>[4x]MVSAPSIDTPSATTFDFDSSVFKKEKVTLSGHDEYIVRGGRNLFPLLPDAFKGIKQIGVIGWGSQAPAQAQNLKDSLTEAKSDVVVKIGLRKGSNSFAEARAAGFSEENGTLGDMWETISGSDLVLLLISDSAQADNYEKVFSHMKPNSILGLSHGFLLGHLQSLGQDFPKNISVIAVCPKGMGPSVRRLYVQGKEVNGAGINSSFAVHQDVDGRATDVALGWSIALGSPFTFATTLEQEYKSDIFGERGILLGAVHGIVECLFRRYTESGMSEDLAYKNTVECITGVISKTISTKGMLALYNSLSE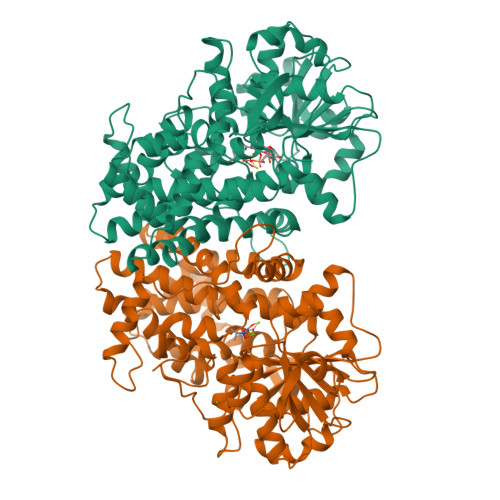EGKKDFQAAYSASYYPSMDILYECYEDVASGSEIRSVVLAGRRFYEKEGLPAFPMGKIDQTRMWKVGEKVRSVRPAGDLGPLYPFTAGVYVALMMAQIEILRKKGHSYSEIINESVIEAVDSLNPFMHARGVSFMVDNCSTTARLGSRKWAPRFDYILSQQALVAVDNGAPINQDLISNFLSDPVHEAIGVCAQLRPSVDISVTADADFVRPELRQA> MTISADISLHHRAVLGSTMAYRETGRSDAPHVLFLHGNPTSSYLWRNIMPLVAPVGHCIAPDLIGYGQSGKPDISYRFFDQADYLDALIDELGIASAYLVAHDWGTALAFHLAARRPQLVRGLAFMEFIRPMRDWSDFHQHDAARETFRKFRTPGVGEAMILDNNAFVERVLPGSILRTLSEEEMAAYRAPFATRESRMPTLMLPRELPIAGEPADVTQALTAAHAALAASTYPKLLFVGSPGALVSP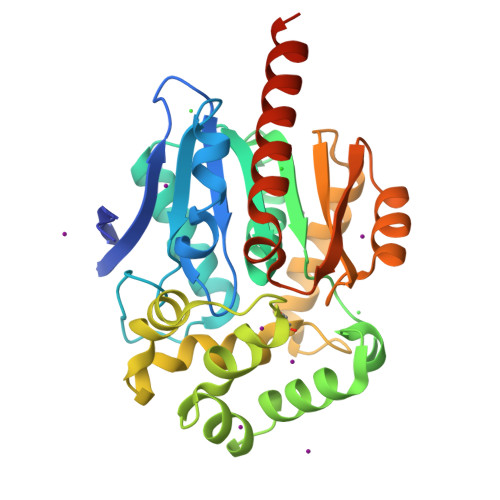AFAAEFAKTLKHCAVIQLGAGGHYLQEDHPEAIGRSVAGWIAGIEAASAQRHAALEHHHHHH> MGSSHHHHHHSSGRENLYFQGMYNTISITVVDADD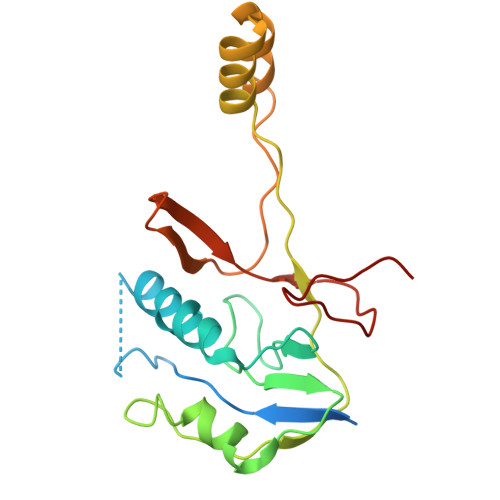VGVNFVVSKVLSTLHNKGIFNGEVGVTFPRMDKNVGDIITLFSKTGVDRKVLTSTLNTLTDFIHIGKPKEADKVKTYRKVDTKSKGKLIRRCIKRKGVSAETAESLYGNYKGEKCKLPYIVVNSKSTGQRFSMFLEECENSEKFNSYGLCIVSC> GETGQVIKSAVRSTVENTVQ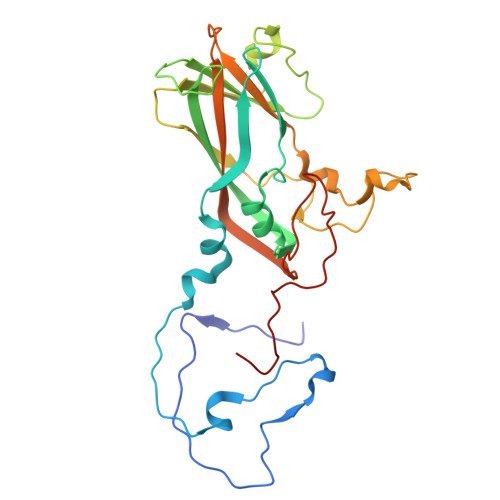STHSITTEATPALQAAETGATSNASDESMIETRNVVNTHGVAETSLEAFYGRAGLVAMFSTDGGIYRWYINFGEYVQLRAKLELLTYARFDMEFTIVAQVVNAQSKVQDFNVDYQVMFVPPGASVPENQDSYQWQSSCNPSVISNTGLPPARVSVPFMSSANAYSFSYDGYTQFGDASGSSYGIVPSNYLGMLVVRTCEDLDGTRLRVRVYAKPKHVKGWIPRSPRMTPYKSRYTGVYTDTTKFCANRARITTAG>GSHMSAELEIDVKTRILDAAADAFMVHGFANTTIDDIAEQVGATKGLIYYHFRSKFDIFLAVYEDGMRRVRERVEPHAGGAGTGRERLVAMSVAHLENLMTELGYHHVVHQGVRYQASTALKIRQRDALAALNELRRDYELMFRRVVAEGIADGSLRVVDEALATRT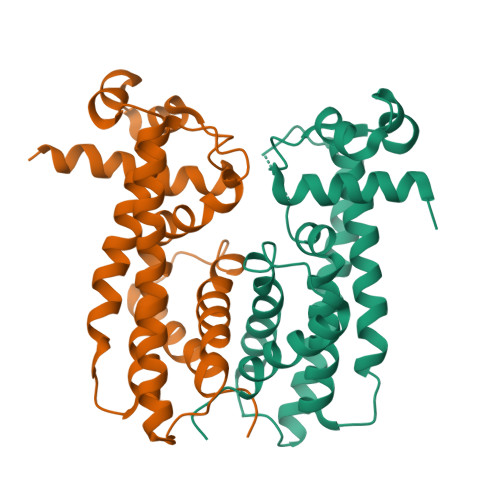LLSNLNAVDMWYRRIEGQTLDEINELATNVVDLLITGMANPQGRPR[4x]> KPEPTDEEWELIKTVTEAHVATNAQGSHWKQKRKFLPEDIGQAPIVNAPEGGKVDLEAFSHFTKIITPAITRVVDFAKKLPMFCELPCEDQIILLKGCCMEIMSLRAAVRYDPESETLTLNGEMAVTRGQLKNGGLGVVSDAIFDLGMSLSSFNLDDTEVALLQAVLLMSSDRPGLACVERIEKYQDSFLLAFEHYINYRKHHVTHFWPKLLMKVTDLRMIGACHASHFLHMKVECPTELFPPLFLEVFE;> ENALLRYLLDK

The thyroid hormone receptors (THRs) are nuclear hormone receptors regulated by endogenous thyroid hormones, including the inactive prohormone thyroxine (T4) and the bioactive hormone 3,3′,5-triiodothyronine (T3), which are critical for development regulation and metabolic homeostasis. As ligand-regulated nuclear receptors, THRs have a structurally conserved LBD that allows the binding of distinct ligands (Burris et al., 2013). Following the ligand binding, the function of THRs is mediated through the selective recruitment or release of specific coregulators, like the family of steroid receptor coactivators (SRCs) (Li et al., 2003, Jin and Li, 2010, Savkur and Burris, 2004), as a heterodimeric complex with retinoid X receptor (RXR) (Putcha et al., 2012, Kojetin et al., 2015, Mangelsdorf and Evans, 1995). Although the defects in any of the processes in thyroid hormone transport and synthesis can all contribute to RTH, in most cases the disorder involves defective thyroid hormone receptors, resulting in reduced T3 binding and disruptive thyroid hormone signaling.

As expected, the native ligand T3 abolished or substantially diminished the transcriptional activity of four THRβ mutants associated with thyroid hormone resistance, V264D, H435L, R438H, and R438W, respectively (Wakasaki et al., 2016, Nomura et al., 1996, Sabet and Pallotta, 2011, Narumi et al., 2010). Surprisingly, the treatment of roxadustat either enhanced or retained the transcriptional activity of these THRβ mutants, all leading to higher induced transcriptional activity than those of T3. In contrast, the binding of roxadustat resulted in higher Tm values for four TRβ mutants than that of T3. Although all four mutant residues are located in the THRβ LBD, H435 is the only one that directly contacts ligands T3 or roxadustat, whereas the rest of the mutant residues are located outside the ligand-binding pocket, not in the range to form intimate contacts with the ligands, which makes us wonder how these mutants influence the ligand binding. To unravel the molecular basis for the RTH of the THRβ mutants and further their beneficial susceptibility to roxadustat, we performed structural studies on the THRβ mutants complexed with roxadustat. The structural analysis further revealed an apparent conformational change of residue H435 on helix 10 of THRβ for all four mutants, resulting in the loss of a critical hydrogen bond between THRβ and a critical hydroxy group of T3, which is also conserved for the other THR ligands identified so far, explaining the severely reduced THRβ activity by T3. Specifically, in addition to the direct mutation of H435 to the hydrophobic leucine of THRβ H435L, the allosteric conformational changes of THRβ H435 were coupled with several intermediate structural changes, predominantly in helix 10, which were initiated by mutants R438H, R438W, or V264D, consequently leading to impaired T3 binding.(2R)-5-{[(2S,3R)-4-{[1-(3-tert-butylphenyl)cyclohexyl]amino}-1-(3,5-difluorophenyl)-3-hydroxybutan-2-yl]amino}-2-hydroxy-5-oxopentanoic 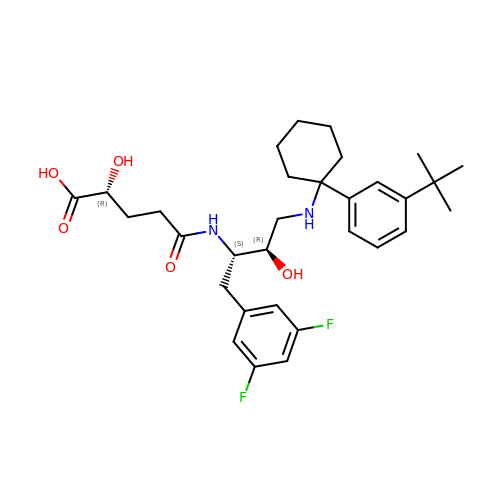acid | C31 H42 F2 N2 O5 | ZQBAKJWCBZPMKW-OYUWMTPXSA-N>[2x]MASGMIVTDAGADQPI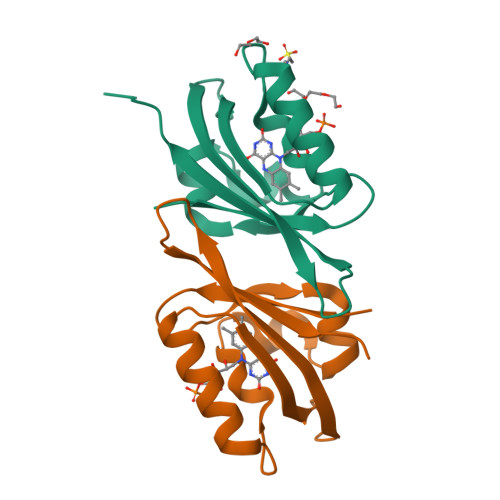VFVNRAFSTITGYAPNEVLGRNARFLQGPQTDAATVARLREAIAAARPIQERILNYRKDGQPFWNQLSISPVRDETGNVVAFVGVDTDVTAHHHHHH>MGSSHHHHHHENLYFQGGCGIGKEAEVKKSFEKTLSMYPIKNLEDLYDKEGYRDDQFDKNDKGTWIINSEMVIQPNNEDMVAKGMVLYMNRNTKTTNGYYYVDVTKDEDEGKPHDNEKRYPVKMVDNKIIPTKEIKDEKIKKEIENFKFFVQYGDFKNLKNYKDGDISYNPEVPSYSAKYQLTNDDYNVKQLRKRYDIPTSKAPKLLLKGSGNLKGSS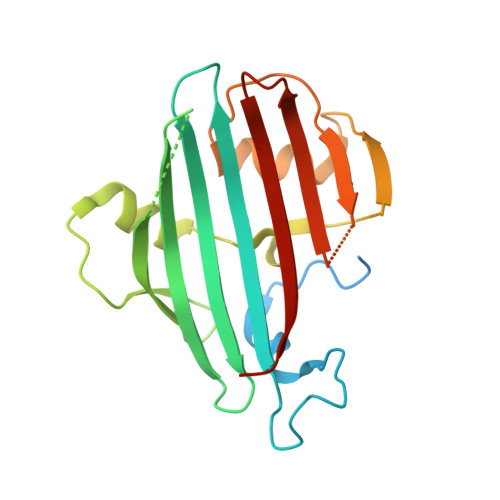VGYKDIEFTFVEKKEENIYFSDSLDYKKSGDV[4x]> CG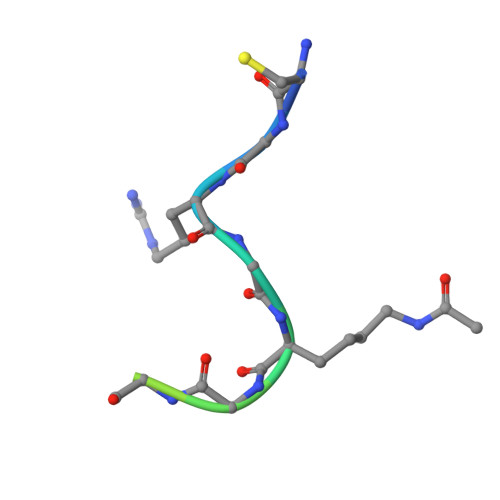RGKGGKGLGKGGA DODECYL NONA ETHYLENE GLYCOL ETHER | C30 H62 O10 | 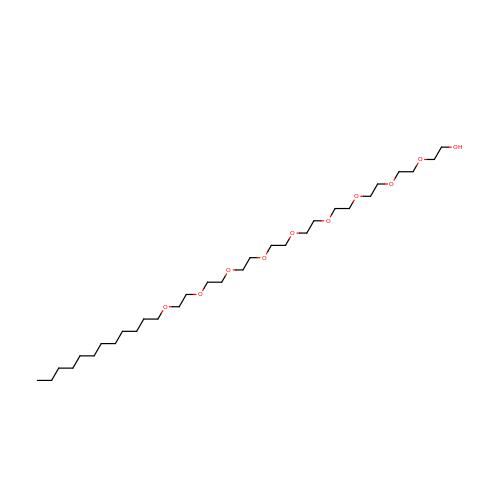ONJQDTZCDSESIW-UHFFFAOYSA-N> MSLPSNPTPVIPANLDLGGINHSAVANRYRNLTKEAQQNLYQF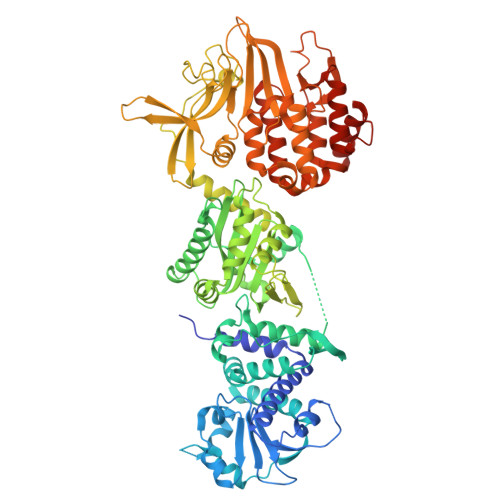AIIEVLSQIREERPDKNLDAYNALIGIDKVTTVDIYTYGATNMFFMPDARGSKTGILVNLNSPDKPYTNIQQPSDFNNINDESFRQNFTSWEKRDGTTYSGVDTALDGLQEGQGGWNLGYFNQKTPRTINISELSKILVERLDYHVSQENNDDQILSTLLLDVLPRSAKGAAREPLGVSASGIPFQLEFTFEGFTSPTDELRAIQSPFSHLAKYFDLLVASTNGSDLQDVEYSQEQAENIGAWIDSGTQLLMSASGIGAAVSVIQGAAGLTADAIEGKEIDPLDVISLSLAAIPGGKIVAKLSKVSKNLGQVVRGGISIAETGVDIVGSSRDLIEGFKKGNFTDIINGLVSVASSSASGRPGKSKIGNAIKKGNPDAPLPTRPTYRNHEGEVRPIPTAQTKSFFERVAIVRREGLSGRGAIGLDLTAAQKRGAELSGMGGTISKSNPNGNVSQVYINEAEGIEKNITYRKVPVPNEPGNFENRLQESFLDNNGQTKWRDFPYAGEEFDFRLQHKDDFNNIGDLGVGKQGIIAVNNPYSFVHHSHTFEQKGISNNHLTLESNAFLTYIEGKKTGDFENKYGNEMEWLVRKFKTKKNDFDLKDIPDNIHFRTDREKGDHSLTTYTLQDFITVVENAPTKMRKVKNDEFALNNIVESMRATAKNMGASPDTLFLDVASTNYMTQLMGQVLTNGRQELNLQGLSNAAQKLRNGASSSV>MGSSHHHHHHHHHHHHSENLYFQGGQYMPNGWQVPAYGMYGQAWNQQGFNQTQSSAPWMRPNYGVQPPQGQ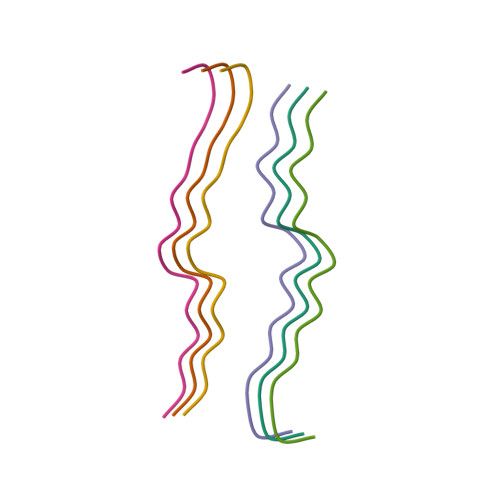NGSMLPNQPSGYRVAGYETQ[6x]> MTVFRQENVDDYYDTGEELGSGQFAVVKKCREKSTGLQYAAKFIKKRRTKSSRRGVSREDIEREVSILKEIQHPNVITLHEVYENKTDVILILELVAGGELFDFLAEKES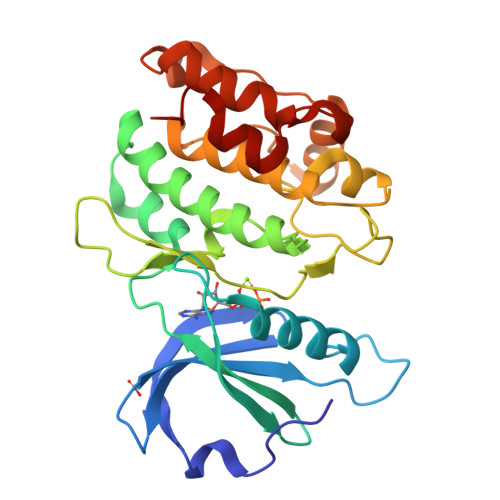LTEEEATEFLKQILNGVYYLHSLQIAHFDLKPENIMLLDRNVPKPRIKIIDFGLAHKIDFGNEFKNIFGTPEFVAPEIVNYEPLGLEADMWSIGVITYILLSGASPFLGDTKQETLANVSAVNYEFEDEYFSNTSALAKDFIRRLLVKDPKKRMTIQDSLQHPWIKP> VTADAALEPDERAAWLAYNDTAEDFPGPHLLARLDAVAREHPDRPAVHAVDGVWTYRELHRRADAVAA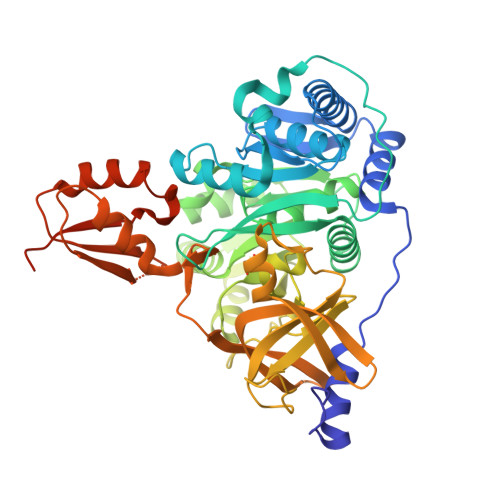FLAARGVRPGSVVAIAATRALAPYAALLGVLKAGCAYVPVNPDDPADRVAFVLADAGATPLLLDTDPASLPAAPAPDVPHEPDRVCYVIYTSGSTGRPKGVVMAERAVDNLTHWVVRRHDVRPDDRLGQTAPLTFDPSVQQVFPAWATGACLVTVPDDVQRDPAAFLDWLRAERVTHLDLVTSHWVHLLNAAEARPAELPDLRWIIIGGETYYYHQTHRWHRVVSSPARLNTIYGPTEAAVNATEHLTEPDLDHGQVPIGVPLPNYRLYALDDDGRLCPPGITGEIHIAGAGLARGYRSAEATAKAFHELEVHSGRTERLYRTGDLARLVRHADRWALEFQGRVDSQVKISGYRVELEEVDAAVKAVPGVRDAAVVVRGEPAEQLVCCYVGDVPPDRLRSRLTERLPAYLVPHLLVPVEALPFTRNGKMDTAELAELVRRFARDS> AAFTQAPMLEQNKQLPPVDQRLPEKPLVIKPIASNGVYGGTLRTVMRGNADGNGILRTIGPQGLTHWTQDIQTVEPYVAESYTVSPDAMEYTFKLRKGMKWSDGTPFTADDIVFAMNDVVLNKEMFPQTPSAYLVGGKAPKVSKVDDYTVKFEFPAANLSFPETLATPLGQHPTLYQKKYCSQFHPAYNKNVQAEFTKANVKDWPSLMRAKCSDIELPSRWSSTERPSIDPWLIKEPYGGAVTRVVMERNPFYWQVDPTGKQLPYVDRIQYAVVSDLQAIILAATNGQYDIEARLLGSDVTSRPLMLKNQQKGGYKVFGQTSANANAAGLWLNQTTKNEKLRKYMTQHD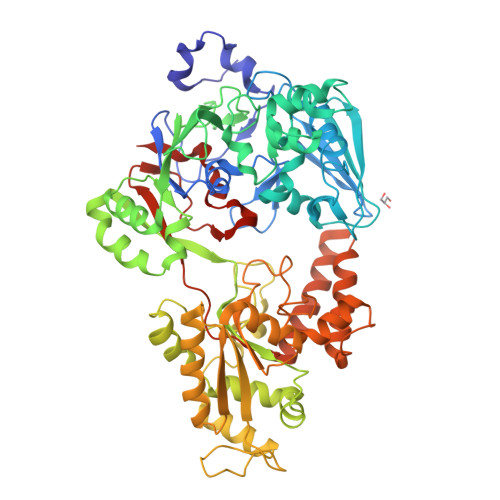FRQALSLAMDRDEINKVAWLGQAAPWQSGPFKESKWYNEKLATQYLKLDLAQANQILDRLGLTKRDSDGYRTYPDGGRVSLDAIVMIDRQAMVQTLELIRRQWQKAGVELVIKGSERSLFYNRATANDYDISIDVFPGGLDATLNPRAYVAVHPLESRMSLEWAKWYLSGGKQGIEPNESMKKRMALYDQFVAAKTQSQALSLFKQILQISADEFEVIGTVRPAVISSLHSLKLQNVNEKMPFGWPYATPSLSLPQQWYFSKLEHHHHHH>SMSSSSRYVTFEGSRNFRLRVVMATLSGKAIKIEKIRSDDLNPGLKDYEVSFLRLMEAVTNGSSIEISYTGTTVIFRPGIITGGSYTHQCPNSKPVGYFAEPMLYLAPFSKKKFSILFRGITSSHNDAGIDAIKWGLMPIMEKFGVRECALHTLKRGSPPLGGGEVHLVVDSLIAQPITMHALDKTMISSIRGVSYSTRVSPSLVNRMIDGAKKVLKSASCEVNITADVWRGENSGKSPGWGLTLVAENKQGWRIFSEAIGDAGDVPEDIGASVAYHLLEEISKSGVVGRNQLPLTILYMIIGKEDIGRLRITKDQIDERFVWLLRDIKKVFGTEILLKPVDD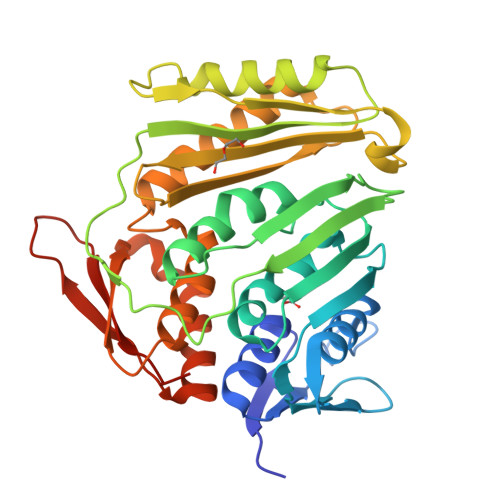NTTDLIATIKGIGFTNTNKKIA[4x]> MWSHPAVRKSSSKTIRSRSIWDDAHAMLEKAKAEGISTVWDRAAEQTPACKFCELGTTCRNCIMGPCRIANRKDGKMRLGVCGADADVIVARNFGRFIAGGAAGHSDHGRDLIETLEAVAEGKAPGYTIRDVAKLRRIAAELGVADAATRPAHDVAADLVTICYNDFGSRRNALAFLARAPQVRRDLWQRLGMTPRGVDREIAEMMHRTHMGCDNDHTSLLVHAARTALADGWGGSMIGTELSDILFGTPRPRQSTVNLGVLRKDAVNILVHGHNPVVSEMILAATREPAVRQAAQDAGAADINVAGLCCTGNELLMRQGIPMAGNHLMTELAIVTGAADAIVADYQCIMPSLVQIAACYHTRFVTTSPKGRFTGATHVEVHPHNAQERCREIVM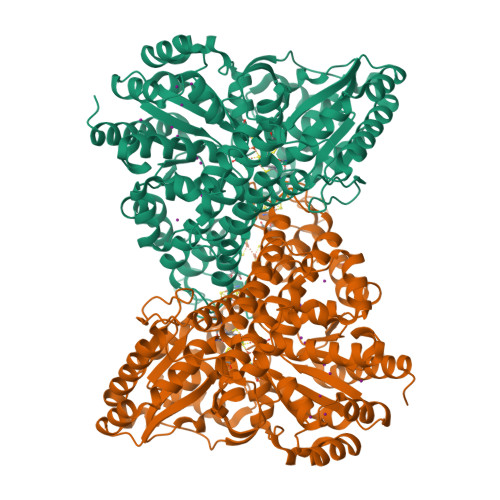LAIDAYTRRDPARVDIPSQPVSIMSGFSNEAILEALGGTPKPLIDAVVAGQIRGFVGIVGCNNPKIRQDSANVTLTRELIRRDIMVLATGCVTTAAGKAGLLVPEAASKAGEGLAAVCRSLGVPPVLHMGSCVDNSRILQLCALLATTLGVDISDLPVGASSPEWYSEKAAAIAMYAVASGIPTHLGLPPNILGSENVTAMALHGLQDVVGAAFMVEPDPVKAADMLEAHIVARRARLGLTS>[2x]EKFLVIAGPNAIESEELLLKVGEEIKRLSEKFKEVEFVFKSSFDKANRSSIHSFRGHGLEYGVKALRKVKEEFGLKITTDIHESWQAEPVAEVAD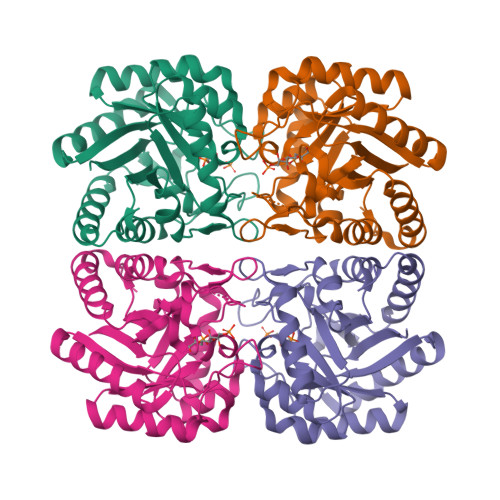IIQIPAFLCRQTDLLLAAAKTGRAVNVKKGQFLAPWDTKNVVEKLKFGGAKEIYLTERGTTFGYNNLVVDFRSLPIMKQWAKVIYDATHSVQLPGGLGDKSGGMREFIFPLIRAAVAVGCDGVFMETHPEPEKALSDAPTALPLSQLEGIIEAILEIREVASKYYETI>[14x]XGEIAKALREIAKALREIAWANRENAKALRGX

αHBs are oligomers of 5 or more α-helical peptides that assemble into coiled-coil structures with central solvent-accessible channels. We targeted two properties of αHBs: oligomeric state, which directly affects the internal diameter of the channel; and the identities of channel-facing residues, which fine tune this dimension and introduce different chemistries. The αHBs are loaded with an environment sensitive dye (in this case, 1,6-diphenyl-1,3,5-hexatriene, DPH) that binds within the channels and fluoresces. Accordingly, challenging the array with analytes leads to differential displacement of the dye across the array to give a fluorescent fingerprint.

Despite the requirements for aliphatic residues at a and d, up to 40% of these can be changed to other side chains without compromising barrel integrity. We introduced mutations at one or two of these sites to generate four groups of αHB: Group I had entirely hydrophobic interiors, but with different sizes and shapes of channel; Groups II and III had polar uncharged or polar charged residues, respectively, at specific points along the channel; and Group IV had aromatic residues installed in their channels. The eleven Group II peptides comprised: single mutants to Cys, His, Asn, Ser or Thr at d sites; and double mutations to His, Asn, Ser or Thr at consecutive a and d sites. Finally, one third of the designs were crystallized and yielded 12 X-ray crystal structures, all of which were open αHBs with fully accessible channels. Focusing on the small molecules, the αSA signal from the more-polar AAs and CHOs is dominated by the polar and charged Group II and III αHBs.>EAPHLVQVDAARALWPLRRFWRSTGFCPPLPHSQADPYVLSWDQQLNLAYVGAVPHRGIKQVRTHWLLELVTTRGSTGQGLSYNFTHLDGYLDLLRENQLLPGFELMGSASGHFTDFEDKQQVFEWKDLVSSLARRYIGRYGLAHVSKWNFETWNEPDHHDFDNVSMTMQGFLNYYDACSEGLRAASPALRLGGPGDSFHTPPRSPLSWGLLRHCHDGTNFFTGEAGVRLDYISLHRKGARSSISILEQEKVVAQQIRQLFPKFADTPIYNDEADPLVGWSLPQPWRADVTYAAMVVKVIAQHQNLLLANTTSAFPYALLSNDNAFLSYHPH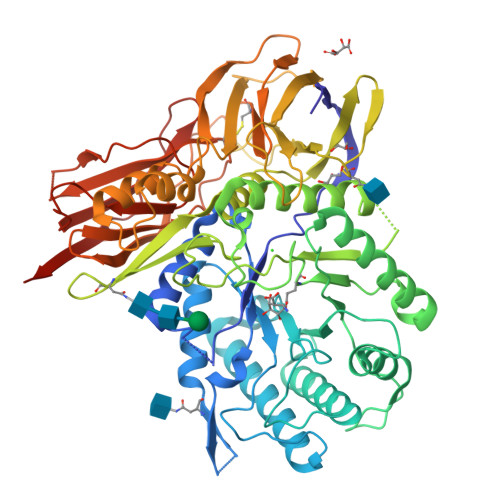PFAQRTLTARFQVNNTRPPHVQLLRKPVLTAMGLLALLDEEQLWAEVSQAGTVLDSNHTVGVLASAHRPQGPADAWRAAVLIYASDDTRAHPNRSVAVTLRLRGVPPGPGLVYVTRYLDNGLCSPDGEWRRLGRPVFPTAEQFRRMRAAEDPVAAAPRPLPAGGRLTLRPALRLPSLLLVHVCARPEKPPGQVTRLRALPLTQGQLVLVWSDEHVGSKCLWTYEIQFSQDGKAYTPVSRKPSTFNLFVFSPDTGAVSGSYRVRALDYWARPGPFSDPVPYLEVPVPRGPPSPGNP[2x]>GMEPRAVADALETGEEDAVTEALRSFNREHSQSFTFDDAQQEDRKRLAKLLVSVLEQGLSPKHRVTWLQTIRILSRDRSCLDSFASRQSLHALACYADIAISEEPIPQPPDMDVLLESLKCLCNLVLSSPTAQMLAAEARLVVRLAERVGLYRKRSYPHEVQFFDLRLLFLLTALRTDVRQQLFQELHGVRLLTDALELTLGVAPKENPLVILPAQETERAMEILKVLFNITFDSVKREVDEEDAALYRYLGTLLRHCVMADAAGDRTEEFHGHTVNLLGNLPLKCLDVLLALELHEGSLEFMGVNMDVINALLAFLEKRLHQTHRLKECVAPVLS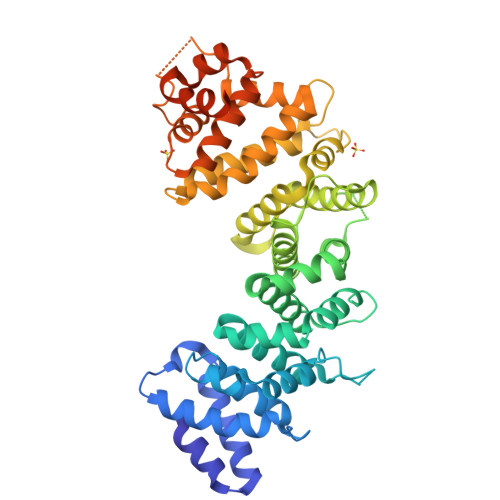VLTECARMHRPARKFLKAQVLPPLRDVRTRPEVGDLLRNKLVRLMTHLDTDVKRVAAEFLFVLCSESVPRFIKYTGYGNAAGLLAARGLMAGGRPEGQYSEDEDTDTEEYREAKASI[2x]S-Trichostatin A | C17 H22 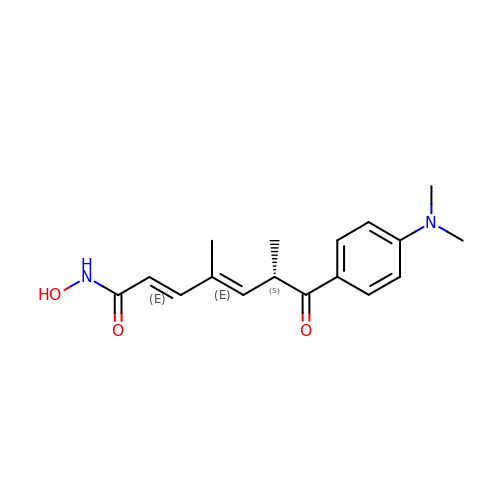N2 O3 | RTKIYFITIVXBLE-LEJRBOCMSA-N>MAPARENVSLFFKLYCLTVMTLVAAAYTVALRYTRTTAEELYFSTTAVCITEVIKLLISVGLLAKETGSLGRFKASLSENVLGSPKELAKLSVPSLVYAV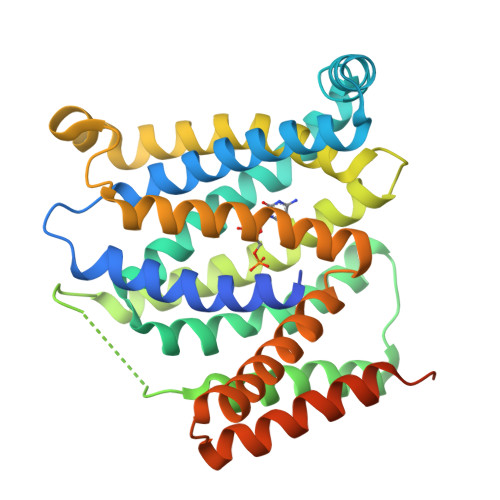QNNMAFLALSNLDAAVYQVTYQLKIPCTALCTVLMLNRTLSKLQWISVFMLCGGVTLVQWKPAQATKVVVAQNPLLGFGAIAIAVLCSGFAGVYFEKVLKSSDTSLWVRNIQMYLSGIVVTLAGTYLSDGAEIQEKGFFYGYTYYVWFVIFLASVGGLYTSVVVKYTDNIMKGFSAAAAIVLSTIASVLLFGLQITLSFALGALLVCVSIYLYGLPRQDTTSIQQEATSKERIIGVSNSLEVLFQ[2x]> ANSRWPTSI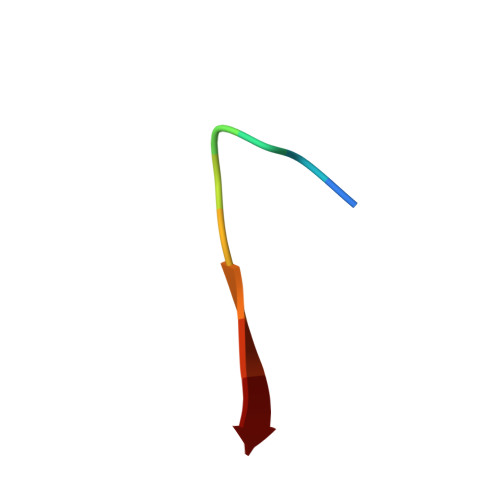I> MTRVVYKVPEEQPPNTLIGSLAADYGFPDVGHLYKLEVGAPYLRVDGKTGDIFTTETSIDREGLRECQNQLPGDPCILEFEVSITDLVQNGSPRLLEGQIEVQDINDNTPNFASPVITLAIPENTNIGSLFPIPLASDRDAGPNGVASYELQAGPEAQELFGLQVAEDQEEKQPQLIVMGNLDRERWDSYDLTIKVQDGGSPPRASSALLRVTVLDTNDNAPKFERPSYEAELSENSPIGHSVIQVKANDSDQGANAEIEYTFHQAPEVVRRLLRLDRNTGLITVQGPVDREDLSTLRFSVLAKDRGTNPKSARAQVVVTVKDMNDNAPTIEIRGIGLVTHQDGMANISEDVAEETAVALVQVSDRDEGENAAVTCVVAGDVPFQLRQASETGSDSKKKYFLQTTTPLDYEKVKDYTIEIVAVDSGNPPLSSTNSLKVQVVDVNDNALEHHHHHH

Protocadherin-1 (PCDH1) is a non-clustered δ1 protocadherin involved in respiratory diseases. PCDH1 has seven EC repeats (labeled EC1 to EC7 from N to C-terminus), a single pass transmembrane domain and a cytoplasmic domain with the three conserved motifs (CM1–CM3) typical of the δ1 subgroup. PCDH1 may bind bronchial epithelial cells and epithelial cells of the airway mucosa together by mediating homophilic adhesion and helping in forming the epithelial barrier. Here we use bead aggregation assays to show that repeats EC1 to EC4 form the minimal adhesive unit for human (Homo sapiens [hs]) PCDH1, despite its longer extracellular domain with seven EC repeats.

The first two, PCDH1 EC3-4bc at 3.05 Å and PCDH1 EC1-4bc at 2.85 Å, were obtained using bacterially produced protein. There are three calcium ions in each complete linker region (EC1–EC2, EC2–EC3, and EC3–EC4) and one calcium ion at the end of EC4. Calcium ions at complete linker regions are coordinated by highly conserved canonical calcium-binding motifs XEXBASE, DXD, DRE/DYE, XDXTOP and DXNDN. An additional calcium ion near the EC2–EC3 linker is unique, it is at a crystal contact, and it might be present due to purification and crystallization conditions with high calcium. Analyses of the interaction interfaces with the Protein, Interfaces, Surfaces and Assemblies (PISA)48 server revealed large interface areas of 1539 Å2 for PCDH1-I1 (385 Å2 per repeat; 486 Å2 for EC1:EC4 and EC4:EC1, 231 Å2 for EC2:EC3 and EC3:EC2) and 1270 Å2 for PCDH1-I2 (423 Å2 per repeat; 461 Å2 for EC2:EC4 and EC4:EC2, 190 Å2 for EC3:EC3) respectively. Both interface areas are greater than 856 Å2, an empirical cut-off to distinguish biological interfaces from crystal contacts. Altogether, these data indicate that the PCDH1-I1 interface mediates trans homodimerization in solution (independently of possible cis dimer conformations induced by C-terminal EC repeats or the Fc tag) and that it is responsible for bead aggregation in vitro.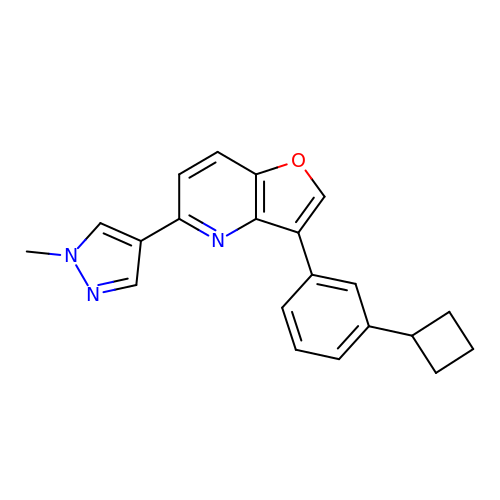3-(3-cyclobutylphenyl)-5-(1-methylpyrazol-4-yl)furo[3,2-b]pyridine | C21 H19 N3 O | DDWOGFZIVMALPO-UHFFFAOYSA-N> INLSNKTDENTISFFDSGDPERMNNEALMRGCGEQIVNLRPLLRTFRTINDNWSLAANTKTPITDLTNTADAEGRDYMSYLSFLYRFYRGGRRYKFFNTTPLKQSQTCYVRSFLIPRNYTADEINTDGPSHITYPVINPVHEVEVPFYSQYRKIPIASTSDKGYDSSLMYYTNVGTQQIVARAGNDDFTFG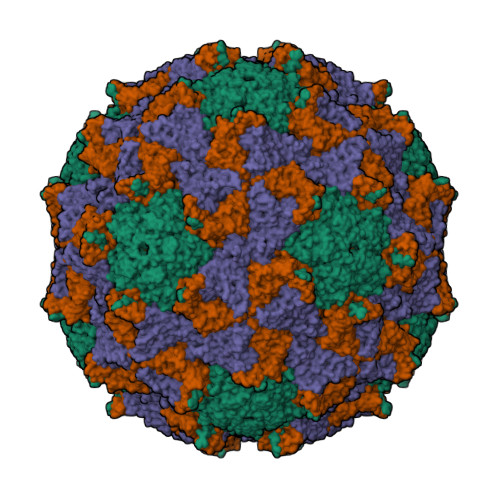WMIGTPQLQGITKEVAN;> ADNQENDSTNVHNTKLASTSAENAIEKEQITTFHDVETPNRIDTPMAQDTSSARSMDDTHSIIQFLQRPVLIDNIEIVAGTTADNNTALSRYVLDRTNPQKYIKQWTLPSTVLKAGGKAQKLANFKYLRCDVQVKIVLNANPFIAGRLYLAYSPYDDKVAPERRIIYTSRAGVTGYPGVELDFQLDNSVEMTIPYASFQEAYDLVSGNEDFVQLYLFTIAPVLGPSAESANSKVDLSVYMWLDNISLVIPTYRLNPNLPTGQTLTRIVQNSDSDKLKEALKIAKSKNPSGYKYIMGVLEQYNPSVKQVSMQ;> SKPRNQNQVMPYQNVPGWGYSLYKGIDMSVPLAYDPNNELGDLRDVFPSAVDEMAIGYVCGNPAIKHVLTWSTTDVVQNPISNGDDWGGVIPVGMPCYSKTIRAVKGATSTSKTEVMDPAPCEYVANLFSYWRATMCYRITVVKTAFHTGRLEIFFEPGSIPTVRTADNLGPDQTQLNGTIAPSDNNYKYILDLTNDTEVTIKVPYVSNKMFMKTVGIYGAHDEDNWNFDESFTGFLCIRPITKLMAPDTVSQKVSIVVWKWAEDVVVVEPKPLTSGPTQVYNPPAVARDLVKQIDVSMQ;> IATPNKSKSTKPTSENPKIGPISEVASGVKTAANGIERIPVLGEIAKPVTAAVKWFADIVGGVAAIFGW>STGMVMVHEVPFPPQIITSKPLSLLGQGITDIEIHFLQVKFTAIGVYLDPSDVKTHLDNWKGKTGKELAGDDDFFDALASAEMEKVIRVVVIKEIKGAQYGVQLENTVRDRLAEEDKYEEEEETELEKVVGFFQSKYFKANSVITYHFSAKDGI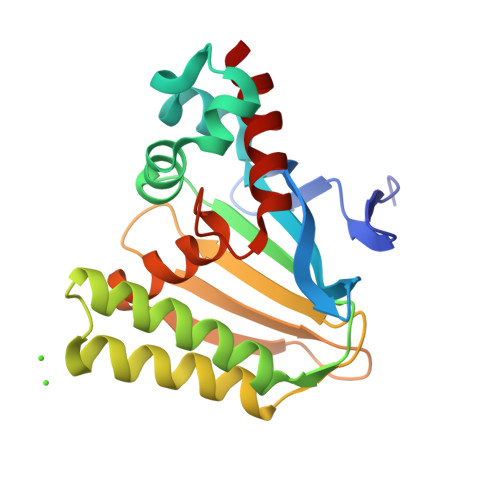CEIGFETEGKEEEKLKVENANVVGMMQRWYLSGSRGVSPSTIVSIADSISAVLT[2x]>[5x]GSHMGGVEVLNIITGPDSTTEIELYLEPRMGINSPTGDKKEWYGYSEVIHHADGYDNNLLSIQMPQYSCARVQLPMLNTDMTSDTLMMWEAVSCKTEIVGIGSLISVHLLEAKMAAKEGGDGPSQPIEGMNYHMFAVGGEPLDLQGIESNALTKYASAIPPKTIHPNDIAKLAEEEKPQLQGLVPKAKARLDKDGFYPIEEWSPDPSRNENSRYFGSFVGGLNTPPNLQFTNAVTTVLLDENGVGPLCKGDGLFVSAADICGVMVKADNEAIRYRGLPRYFKVTLRKRAVKN

Polyomaviruses are small double-stranded DNA (dsDNA) viruses with a circular genome of approximately 5,000 bp. All glycan-binding polyomaviruses analyzed to date engage oligosaccharide (glycan) structures featuring terminal sialic acids that in mammals are usually presented either on gangliosides, which are molecules composed of a glycosphingolipid, i.e., a ceramide and an oligosaccharide, or on glycoproteins, which contain mostly complex and branched oligosaccharides attached to amino acids during co- and posttranslational modification steps. These sialylated glycan structures interact with loop regions at the outer margin of the major capsid protein VP1, at the apical surface of the polyomavirus capsid, as revealed by X-ray crystallography and cryoelectron microscopy. The VP1 surface exhibits an astonishing plasticity, providing virus-specific interactions for a range of Neu5Ac linkage types and further specific characteristics of Neu5Ac-containing glycans.

As the Neu5Ac-binding site residues of NJPyV are highly conserved in ChPyV VP1, we hypothesized that this virus is also able to bind 3′SL. In order to define the ligand binding properties of ChPyV, we solved the unliganded structure of its VP1 pentamer at 1.9 Å resolution. With an RMSD of about 0.5 Å, the ChPyV VP1 monomer superposes very well with a VP1 monomer of the NJPyV VP1-3′SL complex structure, including the region that binds sialic acid in NJPyV. The putative ligand-binding sites are largely blocked in the ChPyV VP1 crystals, preventing soaking with ligands. Cocrystallization with sialylated glycans did not yield well-diffracting crystals. Therefore, we assessed the binding of ChPyV VP1 to 3′SL by STD NMR spectroscopy and introduced a valine-to-phenylalanine mutation (V78F) (equivalent to amino acid residue V78 of NJPyV) in the putative sialic acid-binding site of ChPyV in order to interfere with potential glycan binding. While the STD NMR difference spectrum of wild-type ChPyV VP1 closely resembles that obtained for NJPyV VP1, no saturation transfer was observed for the V78F mutant. We therefore conclude that ChPyV binds 3′SL in a manner that is identical to that observed for NJPyV. For NJPyV, this is demonstrated in solution by STD NMR spectroscopy of 3′SL binding to ChPyV VP1 and by the structure determination of unliganded ChPyV VP1.> MAASKPVEAAVVAAAVPSSGSGVGGGGTAGPGTGGLPRWQLALAVGAPLLLGAGAIYLWSRQQRRREARGRGDASGLKRNSERKTPEGRASPAPGSGHPEGPGAHLDMNSLDRAQAAKNKGNKYFKAGKYEQAIQCYTEAISLCPTEKNVDLSTFYQNRAAAFEQLQKWKEVAQDCTKAVELNPKYVKALFRRAKAHEKLDNKKECLEDVTAVCILEGFQNQQSMLLADKVLKLLGKEKAKEKYKNREPLMPSPQFIKSYFSSF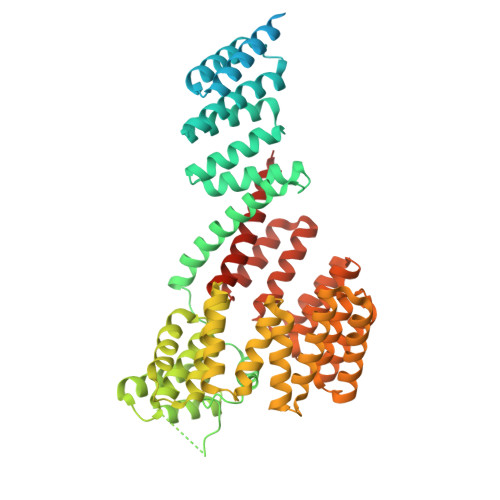TDDIISQPMLKGEKSDEDKDKEGEALEVKENSGYLKAKQYMEEENYDKIISECSKEIDAEGKYMAEALLLRATFYLLIGNANAAKPDLDKVISLKEANVKLRANALIKRGSMYMQQQQPLLSTQDFNMAADIDPQNADVYHHRGQLKILLDQVEEAVADFDECIRLRPESALAQAQKCFALYRQAYTGNNSSQIQAAMKGFEEVIKKFPRCAEGYALYAQALTDQQQFGKADEMYDKCIDLEPDNATTYVHKGLLQLQWKQDLDRGLELISKAIEIDNKCDFAYETMGTIEVQRGNMEKAIDMFNKAINLAKSEMEMAHLYSLCDAAHAQTEVAKKYGLKPPTL> GAMADTCMSRIVKEYKVILKTLASDDPIANPYRGIIES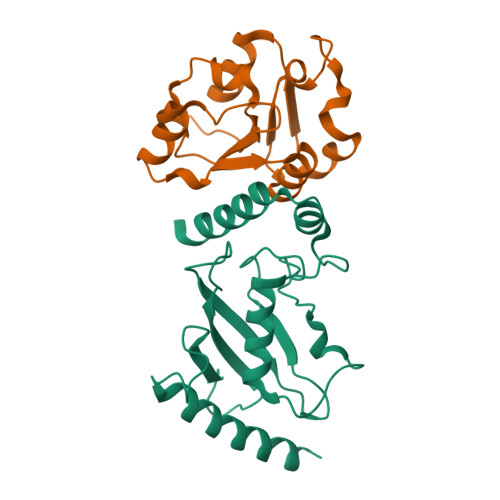LNPIDETDLSKWEAIISGPSDTPYENHQFRILIEVPSSYPMNPPKISFMQNNILHCNVKSATGEICLNILKPEEWTPVWDLLHCVHAVWRLLREPVCDSPLDVDIGAIIRCGDMSAYQGIVKYFLAERERINNH;> GAMENKKARKSKCIIMSKSIQGLPIKWEEYAADEVVLLVPTSHTDGSMKQAIGDAFRKTKNEHKIIYCDSMDGLWSCVRRLGKFQCILNSRDFTSSGGSDAAVVPEDIGRFVKFVVDSDVEDVLIDTLCN>[2x]MLIAVPLDDTNFSENLKKAKEKGADIVELRVDQFSDTSLNYVKEKLEEVHSQGLKTILTIRSPEEGGREVKNREELFEELSPLSDYTDIELSSRGLLVKLYNITK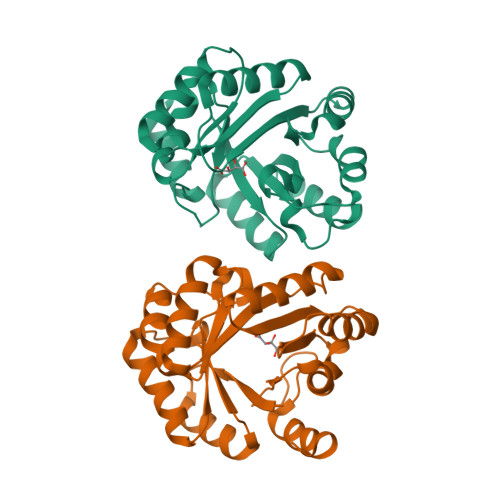EAGKKLIISYHNFELTPPNWIIREVLREGYRYGGIPKIAVKANSYEDVARLLCISRQVEGEKILISMGDYGKISRLAGYVFGSVITYCSLEKAFAPGQIPLEEMVELRKKFYRL> MGSQVSTQRSGSHENSNSATEGSTINYTTINYYKDSYAATAGKQS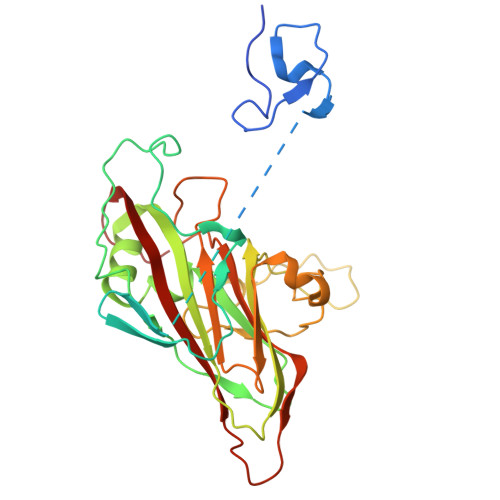LKQDPDKFANPVKDVFTEMAAPLKSPSAEACGYSDRVAQLTIGNSTITTQEAANIIVGYGEWPSYCSDDDATAVDKPTRPDVSVNRFYTLDTKLWEKSSKGWYWKFPDVLTETGVFGQNAQFHYLYRSGFCIHVQCNASKFHQGALLVAILPEYVIGTVAGGTGTEDSHPPYIQTQPGADGFELQHPYVLDAGIPISQLTVCPHQWINLRTNNCATIIVPYMNTLPFDSALNHCNFGLLVVPISPLDFDQGATPVIPITITLAPMCSEFAGLRQAVTQ>[3x]MANCERTFIAIKPDGVQRGLVGEIIKRFEQKGFRLVGLKFMQASEDLLKEHYVDLKDRPWFAGLVKYMHSGPVVAMVWEGLNVVKTGRVM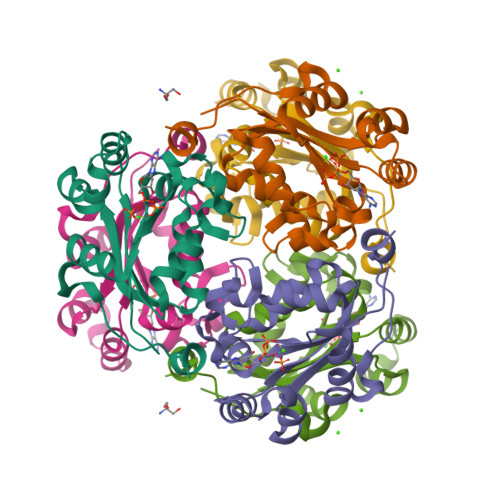LGETNPADSKPGTIRGDFCIQVGRNIIGGSDSVESAEKEIGLWFHPEELVDYTSCAQNWIYE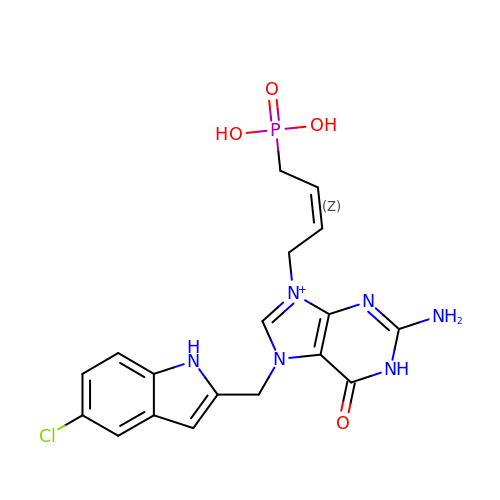[(~{Z})-4-[2-azanyl-7-[(5-chloranyl-1~{H}-indol-2-yl)methyl]-6-oxidanylidene-1~{H}-purin-9-yl]but-2-enyl]phosphonic acid | C18 H19 Cl N6 O4 P | JSTMWLOUXSFOCX-UPHRSURJSA-O> GIGRHTPYGNQTDYRI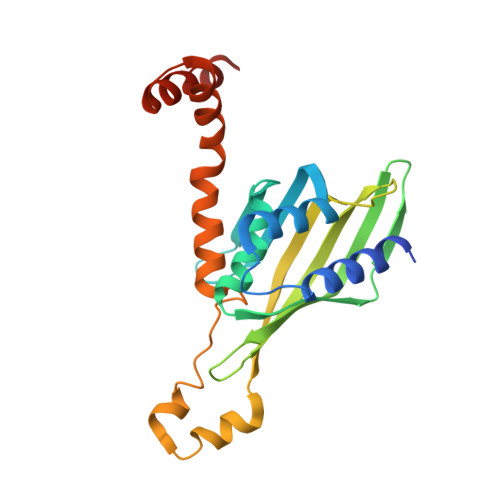FELNKRLQNWTEECDNLWWDAFTTEFFEDDAMLTITFCLEDGPKRYTIGRTLIPRYFRSIFEGGATELYYVLKHPKEAFHSNFVSLDCDQGSMVTQHGKPMFTQVCVEGRLYLEFMFDDMMRIKTWHFSIRQHRELIPRSILAMHAQDPQMLDQLSKNITRCGLSNSTLNYLRLCVILEPMQELMSRHKTYSLSPRDCLKTCLFQKWQRMVAPP> GSMLDGPYQPTTFTPPSDYWILINSNTNGVVYESTNNSDFWTAVIAVEPHVDPVDRQYNVFGENKQFNVRNDSDKWKFLEMFRGSSQNDFYNRRTLTSN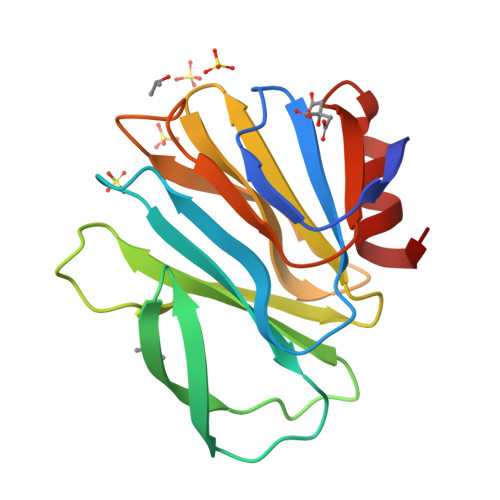TRLVGILKYGGRIWTFHGETPRATTDSSNTANLNGISITIHSEFYIIPRSQESKCNEYINNGL> GSHMEAVQNRIVEAAERVPGVRGVIHLRARYVGQDIWAAMIIGVDPENTVEQAHEICEAVQAAVCGKIRRIESLHVSAEAREIGDTTKPSFSDQPLSFDEVMLSKVDN

One group of metal ion efflux transporters that regulates metal ion homeostasis and can be found in all domains of life is the Cation Diffusion Facilitator (CDF) protein family. One of the most highly conserved and abundant integral MM proteins is the CDF transporter MamM. MamM was recently proposed to function as a magnetosome-directed iron transporter required for iron biomineralization since its deletion abolished magnetite biomineralization and mutation of residues within the conserved TMD metal-binding site resulted in alterations of magnetite crystal size, morphology and even mineral phase. To summarize our results we present an alternative model for the CDF CTD mode of action, in which we propose that upon metal cation binding, the CTD induces conformational changes towards a tighter and more compact fold which allows the activation of iron transport through the TMD.

Examining this closed state model, three putative binding sites were revealed, in which Asp, Glu and His residues from the two monomers are brought into close proximity and may bind divalent cations. The central binding site is presumed to be the main site as it displays tight packing and contains two symmetry-related His285 and two Asp249 residues. The central binding site D249A mutant also displayed a significantly decreased magnetic response that correlated with reduced numbers of magnetite particles per cell (−47%; P<0.001, Mann-Whitney test). Although the average particle size in the cells expressing D249A mutant and in the cells expressing wild-type MamM was similar, the crystal size distribution of the D249A mutant showed a minor shift towards smaller crystals whereas no defects in crystal morphologies were observed. Furthermore, only the D249A and E289A single mutants revealed an additional slight decrease of the magnetic response during iron induction experiments with iron-starved cells. The D249A, H285A and H264A mutants displayed a minor increase in the number of binding sites compared to the wild-type protein, which may be the result of an increased void volume that allowed the accommodation of additional cations after amino acid substitution to alanine. Therefore, the reduced magnetite formation reflects decreased MamM activities caused by less (e.g. MamM D249A) and/or shorter (e.g. MamM D249A+H264A) TMD activation events. To confirm that these observed phenotypic differences are due to true transport function alternations, we also examined the expression levels of all MamM mutants, their ability to stabilize MamB expression, performed MD simulations for dimer stability evaluation and determined their CTD structures. (ii) All mutants exhibited an apo-MamM CTD-like behavior along the MD simulations (see Fig. B in file S1 for representative MD simulations), and (iii) an absence of structural differences was observed.> MT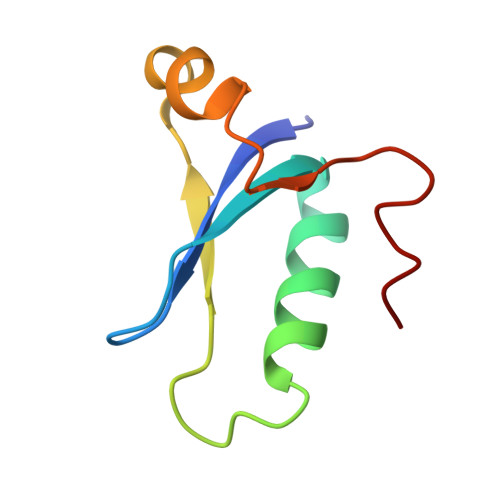SFYKITAYNSQALYFWGTDADVDRYVDWLNRDREINVYAAEAIPEAEWAQYEGRDDVLSGEECGWDDF> ETGTPMMPPVGVQASILSHDTIRITWADNSLPKHQKITDSRYYTVRWKTNIPANTKYKNANATTLSYLVTGLKPNTLYEFSVMVTKGRRSSTWSMTAHGATFELVPTSPPKDVTVVSKEGKPRTIIVNWQPPSEANGKITGYIIYYSTDVNAEIHDWVIEPVVGNRLTHQIQELTLDTPYYFKIQARNSKGMGPMSEAVQFRTPKADSSDKMPNDQALGSAGKGSR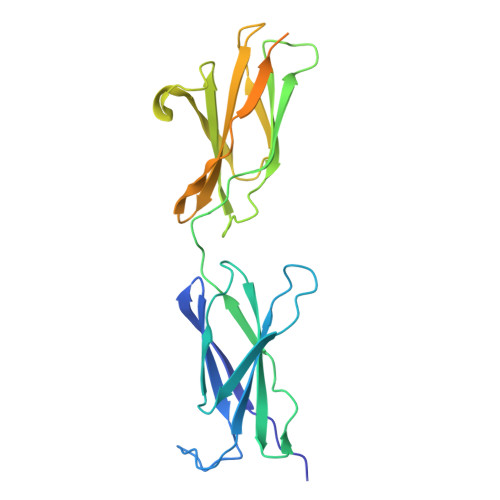LPDLGSDYKPPMSGSNSPHGSPTSPLDSNGTKHHHHHH~{N}-(1~{H}-benzotriazol-5-yl)-2-(2-methylphenoxy)ethanamide | C15 H14 N4 O2 | 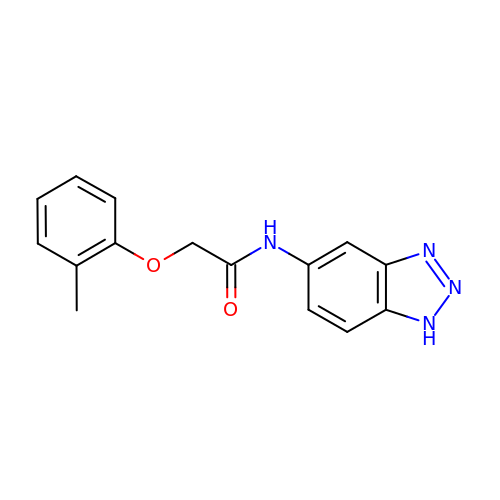VIBQPIOMWNLUQT-UHFFFAOYSA-N> WFGQDGNNYMDIADLHAALQVAPDLDFLFFDACFMEAVEVAYALRDCGSYLISSPTEIPGPGAPYQTVVPAMFSAENAALKIASCYYDYYQSRYDDGIGMSNEDWTGGVSVGVAKMSELENLAVATSKVLPRYITGKQNFDL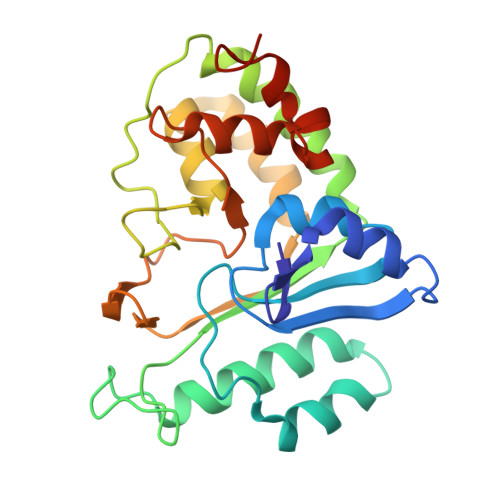SGVMCYDRRTDKQYYYDLDRFIYQITAGNGDYDSWREAFDKVMVYWKSTPRNYSAYAGMFTMNQDAKGLSTYIPRMSAPSLNTSYQQTEWYKVSGWADTGWYKNHHHHHH> DPFAGDPPRHPGLRVNSQKPFNAEPPAELLAERFLTPNELFFTRNHLPVPAVEPSSYRLRVDGPGGGTLSLSLAELRSRFPKHEVTATLQCAGNRRSEMSRVRPVKGLPWDIGAISTARWGGARLRDVLLHAGFPEELQGEWHVCFEGLDADPGGAPYGASIPYGRALSPAADVLLAYEMNGTELPRDHGFPVRVVVPGVVGARSVKWLRRVAVSPDESPSHWQQNDY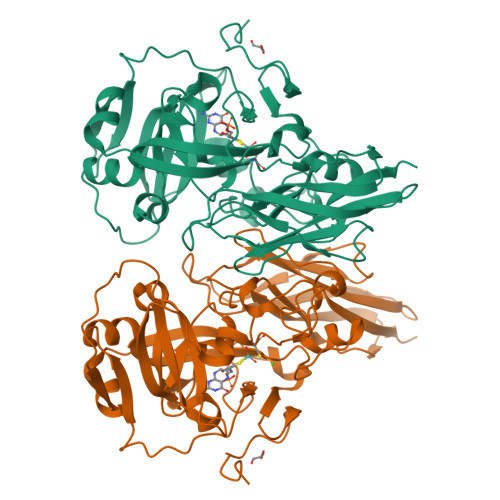KGFSPCVDWDTVDYRTAPAIQELPVQSAVTQPRPGAAVPPGELTVKGYAWSGGGREVVRVDVSLDGGRTWKVARLMGDKAPPGRAWAWALWELTVPVEAGTELEIVCKAVDSSYNVQPDSVAPIWNLRGVLSTAWHRVRVSVQD> 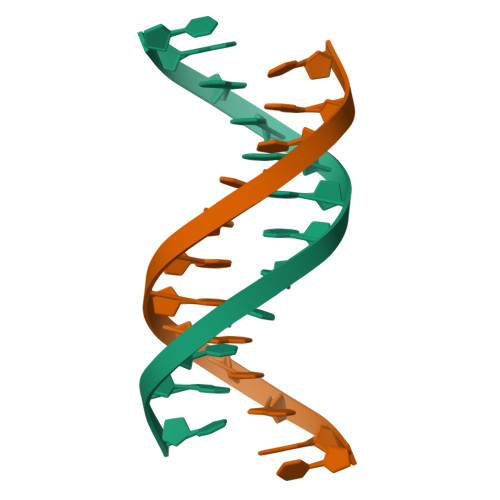CGATATATATAT2-NITROPROPANE | C3 H7 N O2 | 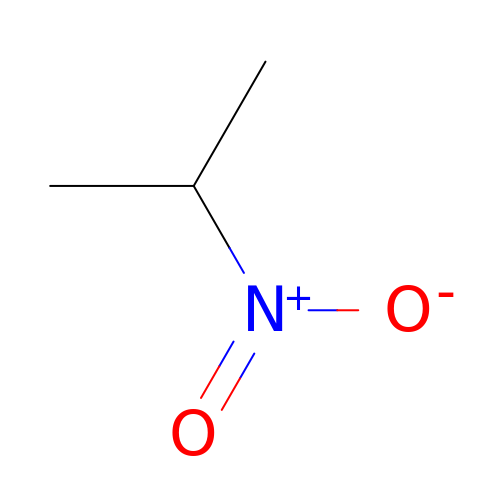FGLBSLMDCBOPQK-UHFFFAOYSA-N> MTSRDGYQWTPETGLTQGVPSLGVISPPTNIEDTDKDGPWDVIVIGGGYCGLTATRDLTVAGFKTLLLEARDRIGGRSWSSNIDGYPYEMGGTWVHWHQSHVWREITRYKMHNALSP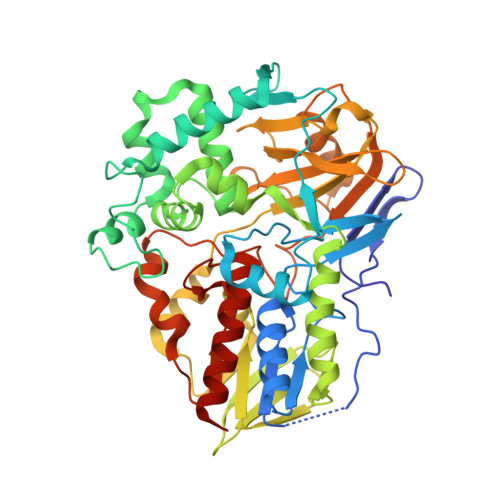SFNFSRGVNHFQLRTNPTTSTYMTHEAEDELLRSALHKFTNVDGTNGRTVLPFPHDMFYVPEFRKYDEMSYSERIDQIRDELSLNERSSLEAFILLCSGGTLENSSFGEFLHWWAMSGYTYQGCMDCLMSYKFKDGQSAFARRFWEEAAGTGRLGYVFGCPVRSVVNERDAARVTARDGREFVAKRVVCTIPLNVLSTIQFSPALSTERISAMQAGHVSMCTKVHAEVDNKDMRSWTGIAYPFNKLCYAIGDGTTPAGNTHLVCFGTDANHIQPDEDVRETLKAVGQLAPGTFGVKRLVFHNWVKDEFAKGAWFFSRPGMVSECLQGLREKHGGVVFANSDWALGWRSFIDGAIEEGTRAARVVLEELGTKREVKARL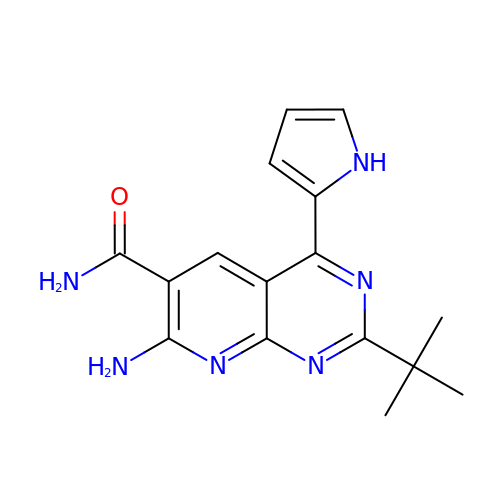7-amino-2-tert-butyl-4-(1H-pyrrol-2-yl)pyrido[2,3-d]pyrimidine-6-carboxamide | C16 H18 N6 O | QZUNGZQACLCXSW-UHFFFAOYSA-N1-[(3S)-1-benzylpiperidin-3-yl]ethanone | C14 H19 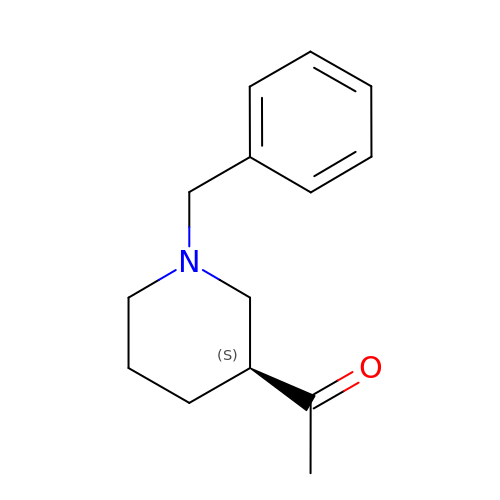N O | PSOOKVRLQJHUPX-AWEZNQCLSA-N9-{5-S-[2-({[(3S)-7-nitro-1,2,3,4-tetrahydroisoquinolin-3-yl]methyl}amino)ethyl]-5-thio-alpha-L-lyxofuranosyl}-9H-purin-6-amine | C22 H28 N8 O5 S | 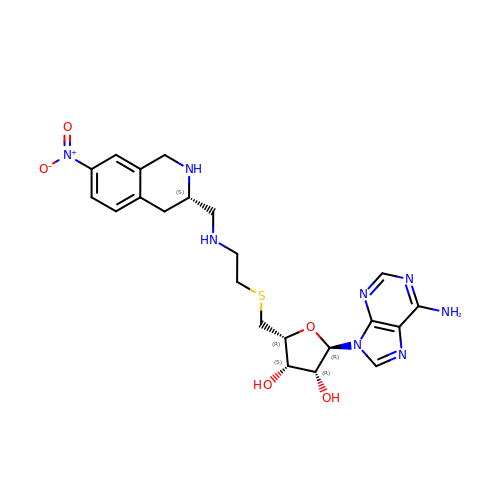XTRSLZMJUJDRCM-RWAFIUBPSA-N> ERLCHPCPWEWTFFQGNCYFMSNSQRNWHDSITACKEVGAQLVVIKSAEEQNFLQLQSSRSNRFTWMGLSDLNQEGTWQW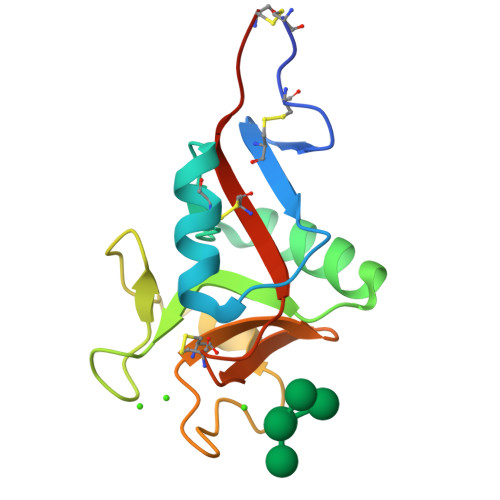VDGSPLLPSFKQYWNRGEPNNVGEEDCAEFSGNGWNDDKCNLAKFWICKKSAASCSRDE> EPSQQ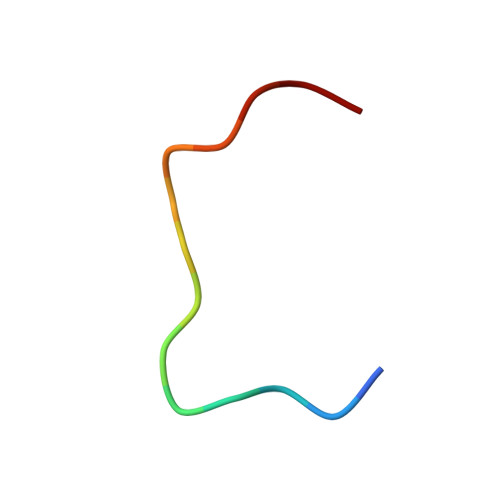VTEIYQHHA2,2-diphenyl-~{N}-[4-(1,3-thiazol-2-ylsulfamoyl)phenyl]ethanamide 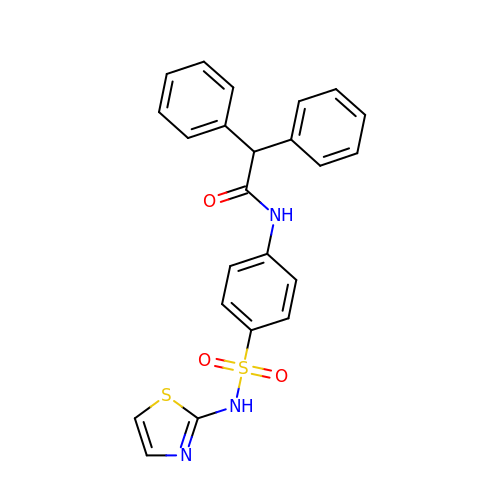| C23 H19 N3 O3 S2 | URSQNPPONHUJDL-UHFFFAOYSA-N> RRRSGSLVYQKRRRRLLPFVSSEDPAQRLKQMGTLASALTELQMEFSDDLTYSSGMAPRSANQARFEEGGMQVLTKEDIETLEQCRAMCKRGDCPPLLVVFDSREGFTVEADGQIKDMTFIAEYTGDVDYIRNREHDDCDSMMTLLLAKDPSSSLVICPDKRGNIARFISGINNHTLDAKKKQNCKCVRYSVNGECRVFL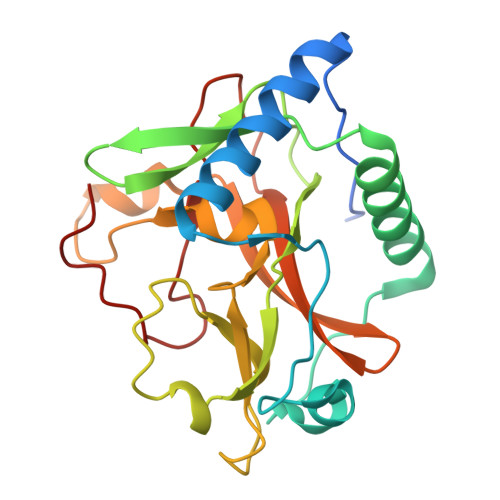VATRDIAKGERLYYDYNGYEHEYPTQHFV> MECPQCGHVSSEKAPKFCSECGQKLPSAATVQGDLKNDNTLVVSSTPEGKTEQGAVLREEEVLLSSTDPGKELEKPEESDSNASWTTQMSKKEKRRRKRQGTISSSEAPSSGLWSLDMPPSPGSHNSALPQNQAQQGGAASQPGHPLDTENMPMEDGFVHTEGSGSPLQGQAAERTDAQSNLAPSDLAEVKDLNTSKPSVDKGLPLDGGPALSAFKGHPKMTDASQKAPLPESKGETSGQEKKVPPIDAAASPVKTAGKETGEDVRKPKPSPVSPVASKHGDQEAELKGKLATPVRKSNEGGNTQPEDQRKPGEGRNFAAAVKTQQAAAPQQAAAPEPTSAFNPRDTVTVYFHAIVSRHFGFNPEEHKVYVRGGEGLGQKGWTDACEMYCTQDLHDLGSLVEGKMDIPRQSLDKPIPYKYVIHRGGSSKDTVEYEFIYEQAQKKGEHVNRCLRVVSTSLGNGDWHQYDDIICMRSTGFFQQAKNRILDSTRKELLKGKKQAAVVMLDRIFSVLQPWSDINLQSFMTQFLQFYSVVREPMIHDGRARKWTSLQYEEKEVWTNLWEHVKKQMAPFLEGKSGESLPADCPVRSKLTLGLSILFMVEAAEFTVPKKDLDSLCYLLIPSAGSPEALHSDLSPVLRIRQRWRIYLTNLCLRCIDERCDRWLGILPLLHTCMQKSPPKKNSKSQPEDTWAGLEGISFSEFRDKAPTRSQPLQFMQSKMALLRVDEYLFRSWLSVVPLESLSSYLENSIDYLSDVPVRVLDCLQGISYRLPGLRKISNQNMKKDVENVFKMLMHLVDIYQHRIFGENLLQIYLTECLTLHETVCNITANHQFFEIPALSAELICKLLELSPPGHTDEGLPEKSYEDLVTSTLQEALATTRNWLRSLFKSRMLSISSAYVRLTYSEEMAVWRRLVEIGFPEKHGWKGSLLGDMEGRLKQEPPRLQISFFCSSQCRDGGLHDSVSRSFEKCVIEAVSSACQSQTSVLEGLSCQDLQKFGTLLSAVITKSWPVHNGEPVFDVDEIFKYLLKWPDVRQLFELCGTNEKIIDNITEEGRQLMATAESVFQKVAGELENGTIVVGQLELILEHQSQFLDIWNLNRRRLPSQEKACDVRSLLKRRRDDLLFLKQEKRYVESLLRQLGRVKHLVQVDFGNIEIIHSQDLSNKKLNEAVIKLPNSSSYKRETHYCLSPDIREMASKLDSLKDSHIFQDFWQETAESLNTLDKDPRELKVSLPEVLEYLYNPCYDNFYTLYENLKSGKITFAEVDAIFKDFVDKYDELKNDLKFMCTMNPQDQKGWISERVGQIKEYHTLHQAVSSAKVILQVRRALGVTGDFSVLNPLLNFADSFEDFGNEKLDQISPQFIKAKQLLQDISEPRQRCLEELARQTELVAWLHKALEDINELKVFVDLASISAGENDIDVDRVACFHDAVQGYASLLYKMDERTNFSDFMNHLQELWRALDNDQHLPDKLKDSARNLEWLKTVKESHGSVELSSLSLATAINSRGVYVIEAPKDGQKISPDTVLRLLLPDGHGYPEALRTYSTEELKELLNKLMLMSGKKDHNSNTEVEKFSEVFSNMQRLVHVFIKLHCAGNMLFRTWTAKVYCCPDGGIFMNFGLELLSQLTEKGDVIQLLGALCRQMEDFLDNWKTVVAQKRAEHFYLNFYTAEQLVYLSSELRKPRPSEAALMMLSFIKGKCTVQDLVQATSACESKADRYCLREVMKKLPQQLLSEPSLMGKLQVIMMQSLVYMSAFLPHCLDLDALGRCLAHLATMGGTPVERPLPKGLQAGQPNLILCGHSEVLPAALAIYMQAPRQPLPTFDEVLLCTPATTIEEVELLLRRCLTSGSQGHKVYSLLFADQLSYEVGCQAEEFFQSLCTRAHREDYQLVILCDAAREHCYIPSTFSQYKVPLVPQAPLPNIQAYLQSHYQVPKRLLSAATVFRDGLCVGIVTSERAGVGKSLYVNTLHTKLKAKLRDETVPLKIIRLTEPHLDENQVLSALLPFLKEKYQKMPVIFHIDISTSVQTGIPIFLFKLLILQYLMDINGKIWRRSPGHLYLVEIPQGLSVQPKRSSKLNARAPLFKFLDLFPKVTCRPPKEVIDMELTPERSHTDPAMDPVEFCSEAFQRPYQYLKRFHQQQNLDTFQYEKGSVEGSPEECLQHFLIYCGLINPSWSELRNFAWFLNCQLKDCEASIFCKSAFTGDTLRGFKNFVVTFMILMARDFATPTLHTSDQSPGRQSVTIGEVVEEDLAPFSLRKRWESEPHPYVFFNGDHMTMTFIGFHLETNNNGYVDAINPSNGKVIKKDVMTKELFDGLRLQRVPFNIDFDNLPRYEKLERLCLALGIEWPIDPDETYELTTDNMLKILAIEMRFRCGIPVIIMGETGCGKTRLIKFLSDLKRGSVEAETMKLVKVHGGTTPSMIYSKVKEAERTAFSNKAQHKLDTILFFDQANTTEAVSCIKEILCDRTVDGEHLHEDSGLHIIAACNPYRKHSQEMILRLESAGLGYRVSAEETADRLGSIPLRQLVYRVHALPPSLIPLVWDFGQLNDSAEKLYIQQIVQRLVDSVSVNPSETCVIADVLSASQMFMRKRENECGFVSLRDVERCVKVFRWFHDHSDMLLKELDKFLHESSDSTHTFERDPVLWSLVMAIGVCYHASLEEKASYRTAIARCFPKPYNSSRAILDEVTHVQDLFLRGAPIRTNIARNLALKENVFMMVICIELKIPLFLVGKPGSSKSLAKIIVADAMQGQAAFSELFRCLKQVHLVSFQCSPHSTPQGIISTFKQCARFQQGKDLGQYVSVVVLDQVGLAEDSPKMPLKTLHPLLEDGCIEDDPAPYKKVGFVGISNWALDPAKMNRGIFVSRGSPNEKELIESAEGICSSDRLVQDKIRGYFAPFAKAYETVCQKQDKEFFGLRDYYSLIKMVFAKAKASKRGLSPQDITHAVLRNFSGKDNIQALSIFTASLPEARYKEEVSTVELIKQNIYPGPQASSRGLDGAESRYLLVLTRNYVALQILQQTFFEGQQPEIIFGSSFPQDQEYTQICRNINRVKICMETGKMVVLLNLQNLYESLYDALNQYYVYLGGQKYVDLGLGTHRVKCRVHTAFRLIVIEEKDVVYKQFPVPLINRLEKHYLDMNTVLQPWQKSIVQELQQWAHEFADVKADQFIARHKYSPADVFIGYHSDACASVVLQAVERQGCRDLTEELYRKVSEEARSILLDCATPDAVVRLSGSSLGSFTAKQLSQEYYYAQQHNSFVDFLQAHLRMTHHECRAVFTEITTFSRLLTGNDCDVLASELRGLASKPVVLSLQQYDTEYSFLKDVRSWLTNPGKRKVLVIQADFDDGTRSAQLVASAKYTAINEINKTQGTKDFVFVYFVTKLSRMGSGTSYVGFHGGLWRSVHIDDLRRSTIMASDVTKLQNVTISQLFKPEDKPEQEEMEIETSQSKELAEEQMEVEDSEEMKKASDPRSCDCSQFLDTTRLVQSCVQGAVGMLRDQNESCARNMRRVTILLDLLNEDNTRNASFLRESKMRLHVLLNKQEENQVRSLKEWVTREAANQDALQEAGTFRHTLWKRVQDVVTPILASMIAHIDRDGNLELLAQPDSPAWVQDLWMFIYSDIKFLNISLVLNNTRSNSEMSFILVQSHMNLLKDAYNAVPFSWRIRDYLEELWVQAQYITDTEGLSKKFVEIFQKTPLGVFLAQFPVAQQQKLLQSYLKDFLLLTMKVSSREELMFLQMALWSCLRELQEASGTPDETYKFPLSLPWVHLAFQHFRTRLQNFSRILTIHPQVLSSLSQAAEKHSLAGCEMTLDAFAAMACAEMLKGDLLKPSPKAWLQLVKNLSTPLELVCSEGYLCDSGSMTRSVIQEVRALWNRIFSIALFVEHVLLGTESHIPELSPLVTTYVSLLDKCLEEDSNLKTCRPFVAVMTTLCDCKDKASKKFSRFGIQPCFICHGDAQDPVCLPCDHVYCLRCIQTWLIPGQMMCPYCLTDLPDKFSPTVSQDHRKAIEKHAQFRHMCNSFFVDLVSTMCFKDNTPPEKSVIDTLLSLLFVQKELLRDASQKHREHTKSLSPFDDVVDQTPVIRSVLLKLLLKYSFHEVKDYIQNYLTQLEKKAFLTEDKTELYLLFISCLEDSVHQKTSAGCRNLEQVLREEGHFLRTYSPGLQGQEPVRIASVEYLQEVARVRLCLDLAADFLSELQEGSELAEDKRRFLKHVEEFCTRVNNDWHRVYLVRKLSSQRGMEFVQSFSKQGHPCQWVFPRKVIAQQKDHVSLMDRYLVHGNEYKAVRDATAKAVLECKTLDIGNALMACRSPKPQQTAYLLLALYTEVAALYRSPNGSLHPEAKQLEAVNKFIKESKILSDPNIRCFARSLVDNTLPLLKIRSANSILKGTVTEMAVHVATILLCGHNQILKPLRNLAFYPVNMANAFLPTMPEDLLVHARTWRGLENVTWYTCPRGHPCSVGECGRPMQESTCLDCGLPVGGLNHTPHEGFSAIRNNEDRTQTGHVLGSPQSSGVAEVSDRGQSPVVFILTRLLTHLAMLVGATHNPQALTVIIKPWVQDPQGFLQQHIQRDLEQLTKMLGRSADETIHVVHLILSSLLRVQSHGVLNFNAELSTKGCRNNWEKHFETLLLRELKHLDKNLPAINALISQDERISSNPVTKIIYGDPATFLPHLPQKSIIHCSKIWSCRRKITVEYLQHIVEQKNGKETVPVLWHFLQKEAELRLVKFLPEILALQRDLVKQFQNVSRVEYSSIRGFIHSHSSDGLRKLLHDRITIFLSTWNALRRSLETNGEIKLPKDYCCSDLDLDAEFEVILPRRQGLGLCGTALVSYLISLHNNMVYTVQKFSNEDNSYSVDISEVADLHVISYEVERDLNPLILSNCQYQVQQGGETSQEFDLEKIQRQISSRFLQGKPRLTLKGIPTLVYRRDWNYEHLFMDIKNKMAQSSLPNLAISTISGQLQSYSDACEALSIIEITLGFLSTAGGDPGMDLNVYIEEVLRMCDQTAQVLKAFSRCQLRHIIALWQFLSAHKSEQRLRLNKELFREIDVQYKEELSTQHQRLLGTFLNEAGLDAFLLELHEMIVLKLKGPRAANSFNPNWSLKDTLVSYMETKDSDILSEVESQFPEEILMSSCISVWKIAATRKWDRQSRGGGHHHHHHHHHH

The giant E3 ubiquitin ligase RNF213 is a conserved component of mammalian cell-autonomous immunity, limiting the replication of bacteria, viruses and parasites. RNF213 is the largest E3 Ub ligase (E3) in the human proteome, combining E3 and AAA (ATPases Associated with diverse Activities) modules into a single ~600 kDa polypeptide. The cryo-EM structure of M. musculus RNF21328 revealed that RNF213 comprises three sub-modules: an N-terminal stalk, a dynein-like AAA core consisting of six ATPase units (only the two units AAA3 and AAA4 can bind and hydrolyze ATP), and a composite E3 module, including a RING domain. Thus, ATP binding to AAA3 and AAA4 subunits is necessary and sufficient to promote the E3 ligase activity of RNF213.

To investigate whether ATPase activity is coupled to E3 activity, we disrupted adenosine-5’-triphosphate (ATP) binding or hydrolysis at the two functional ATPase subunits AAA3 and AAA4 of murine RNF21328. K2387A (WA3) or K2736A (WA4) mutations in the Walker A motifs disrupt ATP binding, whereas isosteric E2449Q (WB3) or E2806Q (WB4) mutations in the Walker B motifs disrupt ATP hydrolysis. Suggestive of O-linked ubiquitination, the Lipid A ubiquitination product was unstable at high pH ( > 10). Together, these data indicate that ATP binding rather than hydrolysis is required to activate the RNF213 E3, regardless of whether the substrate is proteinaceous or non-proteinaceous. Consistent with this, the WB4 mutant underwent robust ABP labeling at ~100-fold reduced ATP levels indicative of sustained RNF213 activation and confirming that ATP hydrolysis counteracts ATP-dependent activation. To enforce an ATP bound state, reasoning this might capture the activated conformation, we determined a structure of the RNF213 WB34 double mutant in the presence of ATP. Structural changes relative to the original ABP-complex were less pronounced (RMSD = 1.57 Å). Although ATP could be modeled into AAA4, AAA3 was empty and once again, there was no clear RZ/Ub density and no clear basis for elevated transthiolating activity. Although we do not elucidate the structural detail of the active site itself, our structure suggests ATP binding induces either long-range allosteric repositioning of the RZ domain, or conformational fine-tuning of the E2-docking CTD, to enable transthiolation from the bound E2~Ub conjugate to the E3 active site. The structural rearrangements that facilitate activation might also be highly transient and recalcitrant to our cryo-EM workflow.> MIKLNCRPLCQTPTASRLV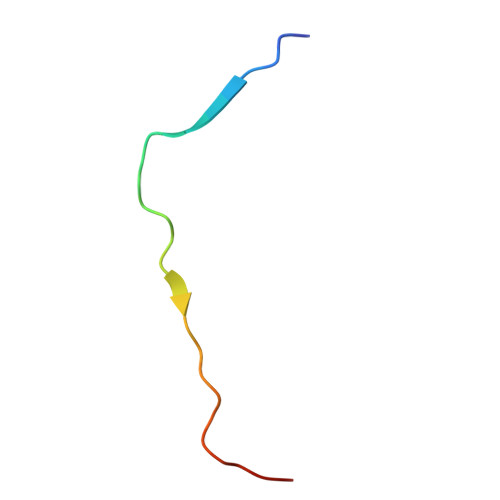SPPCFICRR> AMGSPIFGYSNTQQSQRVVTADNLMYLRSGFAIDAIGTTVNNLVGGPVQGTNGGVLRAPIALDQLQSVEVTSGLYNWGGYHIVAIKFTMKDGSSVLLGSTHYASNKKVETYTVPQGKRIKQINVWTGGWLVEGFQFVY

β-prism folds in V. cholerae are not unique to VCC: three additional β-prism domains exist in two biofilm matrix proteins called RbmC (rugosity and biofilm structure modulator C) and Bap1 (biofilm associated protein 1). RbmC and Bap1 are related multidomain proteins with overlapping functions, involved in the surface attachment of biofilms and encapsulation of growing cell clusters. For simplicity, we refer to the two β-prism domains of RbmC as RbmC1 and RbmC2. Our results illustrate a common structural mechanism by which vibrio toxin and biofilm β-prism domains target glycans on host cell-surfaces, facilitating cell lysis in one case and cell attachment in another.

RbmC2 was crystallized in the presence of N-acetylglucosaminyl-β-1,2-mannose (GlcNAc-Man), and the structure solved to 1.8 Å resolution. Density for the GlcNAc-Man ligand was observed in the same binding pocket identified in the RbmC2/mannotriose and VCC β-prism/methyl-α-mannose complexes. Alternate configurations for the two ligands were built into the density and their relative occupancies were refined, yielding a ratio of 65% GlcNAc-Man to 35% glycerol (presumably from the cryoprotectant). The mannose moiety occupies the same location as the α1,6-linked mannose in the mannotriose structure, making a similar constellation of hydrogen-bonding interactions. Coordination of the disaccharide by RbmC2 resulted in a total of 338 Å2 of buried surface area with a contribution of 160 Å2 by the mannose moiety and 179 Å2 by the N-acetylglucosamine. The N-acetylglucosamine moiety of the GlcNAc-Man structure was observed projecting away from the mannotriose binding cleft. Fewer hydrogen-bonding contacts are made between RbmC2 and this sugar, perhaps contributing to the higher B-factors and less well-defined electron density for this group. In fact, only a single hydrogen bond was observed with the GlcNAc group: between the acetyl O7 atom and the guanidinium group of R876. The only other observed contact between RbmC2 and the GlcNAc moiety is a van der Waals contact between the sugar ring and the side-chain of V874. Interestingly, the centrally located water molecule observed in the mannotriose structure was also present, even though the fourth coordination site (previously made by the central mannose moiety) is missing in this structure.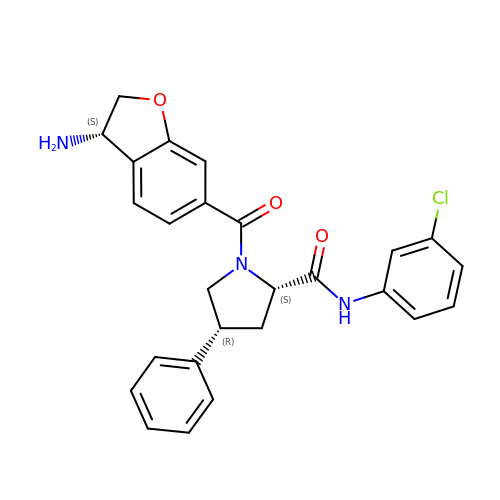(2~{S},4~{R})-1-[[(3~{S})-3-azanyl-2,3-dihydro-1-benzofuran-6-yl]carbonyl]-~{N}-(3-chlorophenyl)-4-phenyl-pyrrolidine-2-carboxamide | C26 H24 Cl N3 O3 | WXCDYJQWHUGJRV-NMNUPHIUSA-N2-[(4-methoxy-2-methyl-phenyl)amino]-7-methyl-9-(4-oxidanylcyclohexyl)purin-8-one 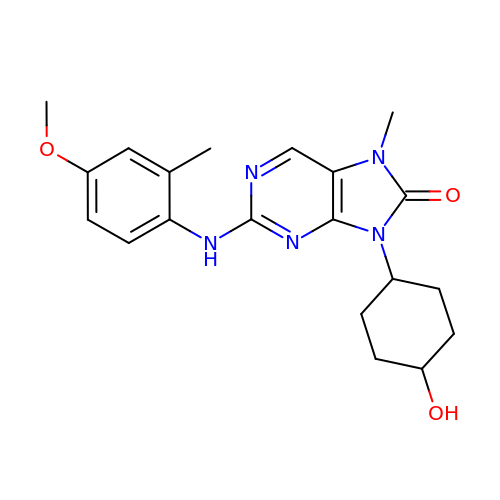| C20 H25 N5 O3 | MFVOIPKDSOFMQO-HDJSIYSDSA-N(2E)-N-hydroxy-3-{4-[(E)-phenyldiazenyl]phenyl}prop-2-enamide 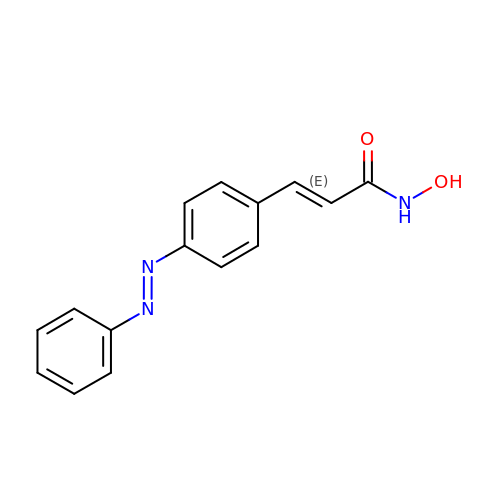| C15 H13 N3 O2 | FBLBOLZQIKQUIK-USZUYCLASA-N acetylsisomicin | C21 H39 N5 O8 | 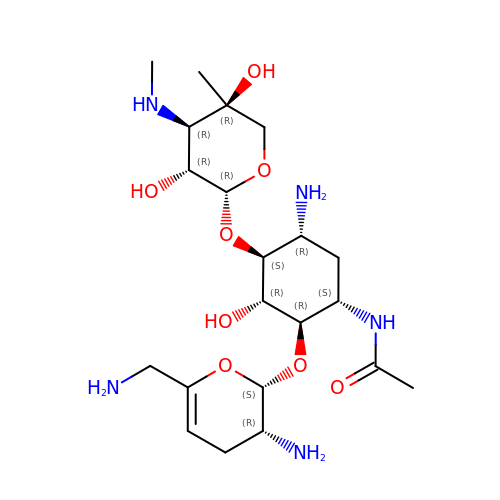OBNIYNLDNPJJOU-IMHCYBRXSA-N> MAHHHHHHVDDDDKMVHHDGFQTVKATIDWEHPMFKLYEKAKRNGKWNPADIDFSQDQKDFASLTSEEKISALPLVAGFSAFEEAVTLDILPMAHALARQGRLEDVLFLTTFMHDEAKHVEMFSRWQQAVGIGQMDLSVFHNDHYKRIFYEALPEAMNRLYADDSPEAVIRAATVYNMIVEGTLAESGYYTFRQIYKKAGLFPGLLQGIDYLNMDEGRHIQFGIYTIQRIVNEDERYYELFIRYMDELWPHVIGYVDYLTELGKRQQQLARTYA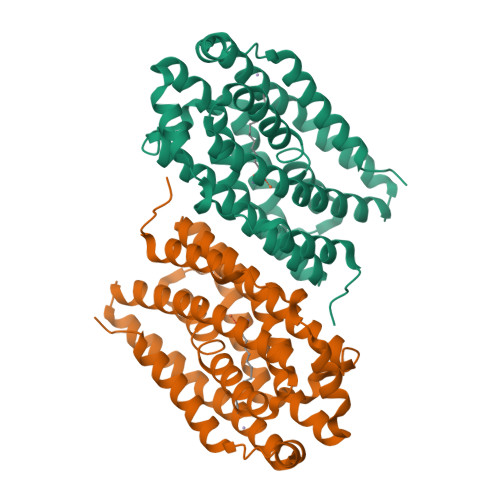LEIDYDLLRHYVIKQFNLRKKQISRTKRVDVVEGLEKTAAES N,N'-(9,10-dioxo-9,10-dihydroanthracene-2,7-diyl)bis[2-(dimethylamino)acetamide] 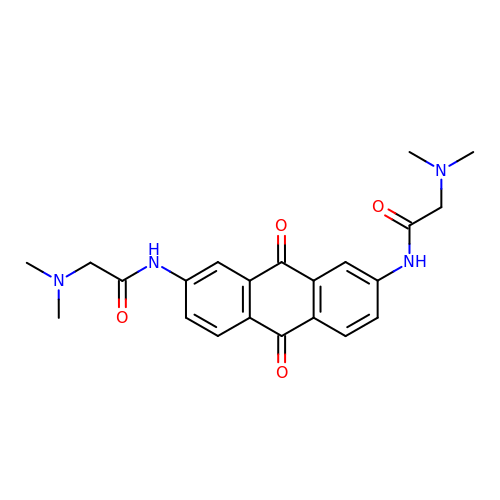| C22 H24 N4 O4 | BQUQDCVNESTXAU-UHFFFAOYSA-N> SMARDYDHLFKLLIIGDSGVGKSSLLLRFADNTFSGSYITTIGVDFKIRTVEINGEKVKLQIWDTAGQERFRTITSTYYRGTHGVIVVYDVTSAESFVNVKRWLHEINQNCDDVCRILVGNKNDDPERKVVETEDAYKFAGQMGIQLFETSAKENVNVEEMFNCITELVLRA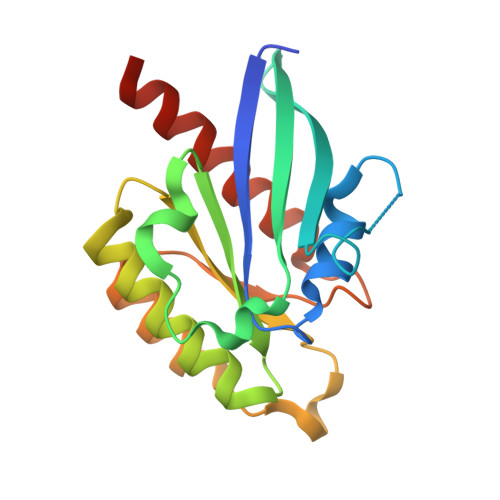KKDNLAKQQ>[2x]METQKLISMVKEALEKYQYPLTAKNIKVVIQKEHN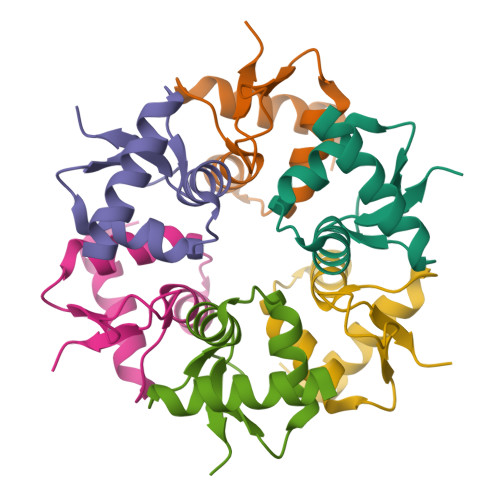VVLPTGSINSILYSNSELFEKIDKTNTIYPPLWIRKN The armadillo repeat serves as a scaffold for the development of modular peptide-recognition modules. In order to develop such a system, three crystal structures of designed armadillo-repeat proteins with third-generation N-caps (YIII-type), four or five internal repeats (M-type) and second-generation C-caps (AII-type) were determined at 1.8 Å (His-YIIIM4AII), 2.0 Å (His-YIIIM5AII) and 1.95 Å (YIIIM5AII) resolution and compared with those of variants with third-generation C-caps. All constructs are full consensus designs in which the internal repeats have exactly the same sequence, and hence identical conformations of the internal repeats are expected.

The crystal structures of His-YIIIM4AII and His-YIIIM5AII were refined at 1.8 and 2.0 Å resolution, respectively. In both cases the asymmetric units contain tetramers with 222 point symmetry and very similar topologies. The quaternary structures of His-YIIIM4AII and His-YIIIM5AII are governed by calcium ions that connect neighbouring chains in a zipper-like manner and the His6 tag that binds to the supposed peptide-binding site, albeit in different orientations (see below). The His-YIIIM4AII tetramer contains 16 calcium ions. The coordination number of each calcium ion in His-YIIIM4AII is seven, which agrees very well with the statistical analysis of calcium-coordination geometry in protein and small-molecule complexes. In contrast to many natural calcium-binding sites, where all coordination bonds are approximately equal in length, the His-YIIIM4AII calcium-binding sites are distorted. In His-YIIIM4AII the axial calcium–ligand distances are shorter than the equatorial distances (axial distances 2.1–2.2 Å; equatorial distances 2.4–3.0 Å) and the Glu25 OE2–Ca bonding distances differ significantly from the average coordination bond length. The His-YIIIM4AII tetramer is further stabilized by interactions between the N-terminal His6 tag and the supposed peptide-binding site. Since all four chains of His-YIIIM4AII are very similar (r.m.s.d. of 0.28 Å for residues 14–246) these interactions are equivalent in all four subunits of the crystallographic tetramer. The structures of His-YIIIM4AII and YIIIM5AII represent extreme cases that are most different.

>[4x]HHHHHHGSELPQMVQQLNSPDQQELQSALRKLSQIASGGDEQIQAVIDAGALPALVQLLSSPNEQILQEALWTLGNIASGGDEQIQAVIDAGALPALVQLLSSPNEQILQEALWTLGNIASGGDEQIQAVIDAGALPALVQLLSSPNEQILQEALWTLGNIASGGDEQIQAVIDAGALPALVQLLSSPNEQILQEALWTLGNIASGGNEQKQAVKEAGALEKLEQLQSHENEKIQKEAQEALEKLQS>MELKQAFVFEFDENLSSSSGSIHLEKVKQNCSPNYDYFKITFIDGYLYIKNKSGVILDKYDLKNVISLVALKRDYLSLSLSNNKQIKKFKNIKNKHLKNKFNLYVINEDIEKRITKNGILEEVILNKMLLSILLGNEENLLQIS[2x];>MQTTTLNWDTVYAVPINIVNEAIKLKHPTPENFELLNGKYGNCSGSFEEWQITNGGDGSNIRLKIPIKNFKATIIGNRLNGKGGFAFANLEVQVKLKYLPHFPQSKNKDIELVDLKIRTQSDNPEDPAIIVISSYKNIQGFYFEDEYKLTEDDEFVVSYFYRLIKEWLEKNLHFFNYIFNTVNLNLYISDK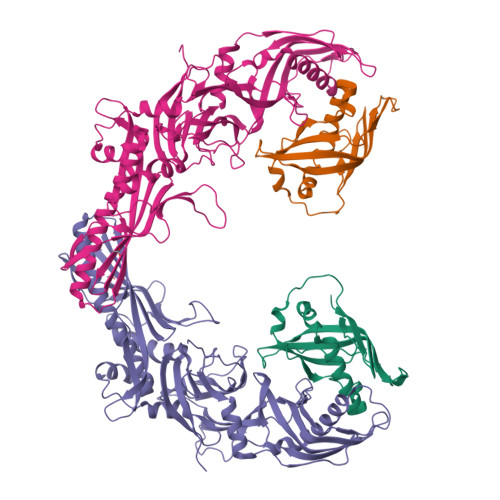EKWEWTKPSYVDYAYSEIEGDLSRSALGVLCMTGGRTGSKNQQQKIDPYAIPAASQSGFLISEERLLRNILLPTIPKKFPKSKGDEFEVINESSQGGGYSYILKLKKGKKIDLENIQAVGYTCTPYIQEMKIYLLGSYLKLETTTRVDLPLGVASICETTCEYKFKLSTNNKGEQTIAYEQIGSPVNIQYSENTGNVGLNIVVSFLSATLSFALTFVPGFGTFLAVGLIGGCLIGSVALIPTFIESYNSDTAPSIDLSLENSVSEITWNSSDVFNLDYVALAGPLQLGGTLQVQNS[2x]Dihydroneopterin aldolase (DHNA) is essential for folate biosynthesis in microorganisms. DHNA catalyzes the conversion of 7,8-dihydroneopterin (DHNP) to 6-hydroxymethyl-7,8-dihydropterin (HP). Without a counterpart in mammals, DHNA is an attractive target for antimicrobial agents. Like other DHNAs, the active site of HpDHNA is formed by catalytic residues from two adjacent subunits in a tetramer.

We have determined the crystal structure of H. pylori DHNA (HpDHNA) in complex with a pterin molecule (HpDHNA:Pterin) at 1.49-Å resolution. The asymmetric unit of the HpDHNA:Pterin structure contains one GGG-DHNA polypeptide, one pterin molecule, one ethylene glycol molecule, and 134 water molecules. The M1-E114 sequence of the HpDHNA protein folds into a four-stranded antiparallel β-sheet (β1, β2, β3, and β4) flanked with three α-helices (α1, α3, and α4). Unlike other DHNAs, the α2 and 310 helices are not observed in HpDHNA apparently due to a six-residue sequence deletion. The HpDHNA:Pterin complex forms a donut-shaped tetramer with four identical subunits related by a four-fold axis. In the tetramer, β1 of each subunit reaches β4 of neighboring subunit with 11 hydrogen bonds, resulting in a sixteen-stranded antiparallel β-sheet in the shape of a perfect barrel wall. The pterin molecule is buried deep in the active site of HpDHNA. It is recognized by the enzyme via π-π stacking with residue Y50 and hydrogen bonding with residues D49, L48, E70, and I69. Although pterin recognition by HpDHNA exhibits common features of ligand binding by DHNAs, the exit of HpDHNA's active site is blocked by residues L21 and I51. The contact distance between L21 and I51 is only 5.2 ​Å.

> GGGMKTKQGVHVHNLVFETILGILEFERLKPQKISVDLDLFYTQLPNKAYLDYIKIQELIQKMMQEKQYLLIEDALKDLSQILKTRYKEITELYLKISKLEISPDSQVGASVKICYENNL> GGELMIKSSNAFDVIELSSQIQRYASLSKINNRTNPILKDNKAKEFKDADLKWLKLENCPTAGDVPTTGNNNDLQDQFIACDADYRKGDLSYFGSQFEFSTYVHPSNPEIQRQIKQVVSYFQYRGMERAFIGDAAGYVISEAKKKGFSAQDYRIVLIEPDRVGYFESNAISYEEFIENPSARENFLLKATKDRTLALAVSLAQTGEIAMQRDGSVAFLEDSELCWDTAAGSAKSCLSVRYDTVGNKTELDLKQIDVVSAKGLSFESDGKTKTPVVSTYETFQDGGRAKTINAIECPTGLNNRFAAVVSSFSTAGQNANFSSESAKDSQGTTQKD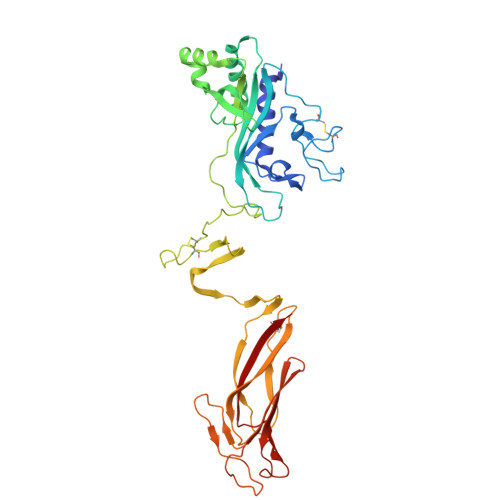GSKGPHALLSGISLNWTLTNKVWDVTASIGIESGILPTSGIDSGSLLRNPKSLSFIAFQWCEN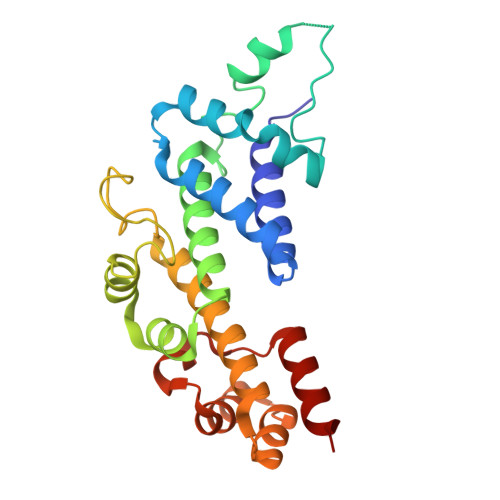>[2x]GPSAKNKEFFDALEEIAESAKNDETLRNELAKVLDDILKTDPSDPEAFRKIVAEHQEFWDEHDPSLMEFNEGRFFGKSRKQYLKSDDFLNSTDPTYNFQKLHQFAAEQRVKLGLEKSDTDTLVAILKNNPEECRAYIESKKPGLGNFSEGNVHGGSGGVLSDEAIKRIKEQARDLLLLKLINSSGNTQLLKDLRDAMSKPEAERAANALGFPTEGNGVLFLSREVVDALEERVEKLA> GPHMACNFQFPEIAYPGKLICPQYGTENKDGEDIIFNYVPGPGTKLIQYEHNGRTLEAITATLVGTVRCEEEKKTDQEEEREGTDQSTEEEKSVDASPNDVTRRTVKNILVSVLPGTEKGRKTNKYANNDFANNLPKEGDIVLTRVTRLSLQRANVEILAVEDKPSPIDSGIGSNGSGIVAAGGGSGAATFSVSQASSDLGETFRGIIRSQDVRSTDRDRVKVIECFKPGDIVRAQVLSLGDGTNYYLTTARNDLGVVFARAANGAGGLMYATDWQM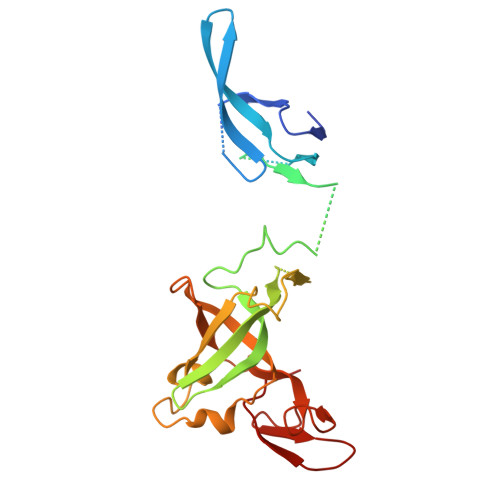MTSPVTGATEKRKCAKPF(1S)-1-(1H-benzimidazol-2-yl)ethyl 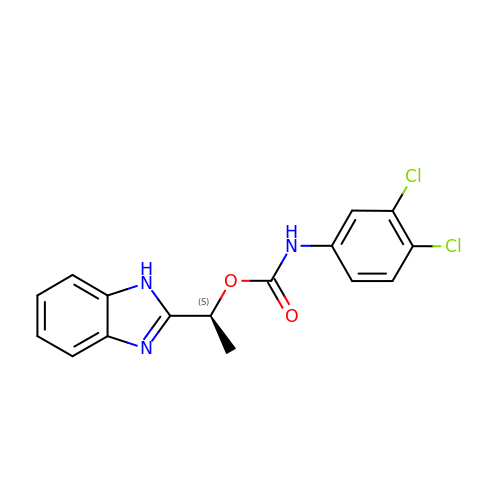(3,4-dichlorophenyl)carbamate | C16 H13 Cl2 N3 O2 | MVMZWHAHBIJEDT-VIFPVBQESA-N> ATVKQPSIGRYTGKPNPSTGKYTVSFIEGDGIGPEISKSVKKIFSAANVPIEWESCDVSPIFVNGLTTIPDPAVQSITKNLVALKGPLATPIGKGHRSLNLTLRKTFGLFANVRPAKSIEGFKTTYENVDLVLIRENTEGEYSGIEHIVCPGVVQSIKLITRDASERVIRYAFEYARAIGRPRVIVVHKSTIQRLADGLFVNVAKELSKEYPDLTLETELIDNSVLKVVTNPSAYTDAVSVCPNLYGDILSDLNSGLSAGSLGLTPSANIGHKISIFEAVHGSAPDIAGQDKANPTALLLSSVMMLNHMGLTNHAD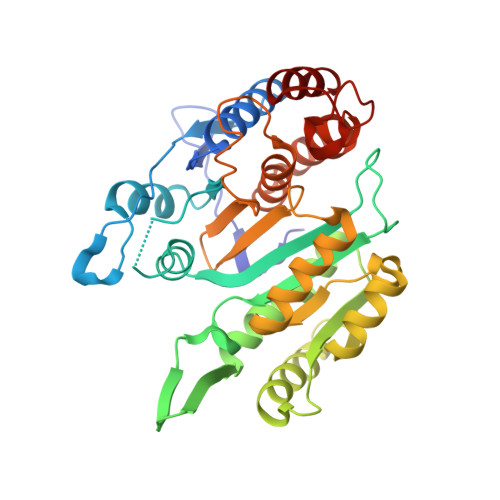QIQNAVLSTIASGPENRTGDLAGTATTSSFTEAVIKRL> IGDEPLENYLDTEYFGTIGIGTPAQDFTVIFDTGSS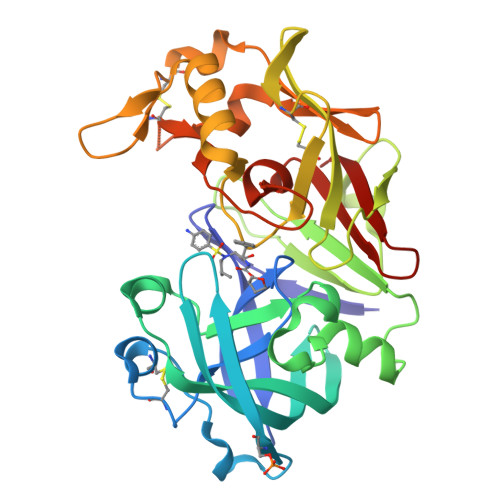NLWVPSVYCSSLACSDHNQFNPDDSSTFEATSQELSITYGTGSMTGILGYDTVQVGGISDTNQIFGLSETEPGSFLYYAPFDGILGLAYPSISASGATPVFDNLWDQGLVSQDLFSVYLSSNDDSGSVVLLGGIDSSYYTGSLNWVPVSVEGYWQITLDSITMDGETIACSGGCQAIVDTGTSLLTGPTSAIANIQSDIGASENSDGEMVISCSSIDSLPDIVFTINGVQYPLSPSAYILQDDDSCTSGFEGMDVPTSSGELWILGDVFIRQYYTVFDRANNKVGLAPVA> AKWVYKFEEGNASMRNLLGGKGCNLAEMTILGMPIPQGFTVTTEACTEYYNSGKQITQEIQDQIFEAITWLEELNGKKFGDTEDPLLVSVRSAARASMPGMMDTILNLGLNDVAVEGFAKKTGNPRFAYDSYRRFIQMYSDVVMEVPKSHFEKIIDAMKEEKGVHFDTDLTADDLKELAEKFKAVYKEAMNGEEFPQEPKDQLMGAVKAVFRSWDNPRAIVYRRMNDIPGDWGTAVNVQTMVFGNKGETS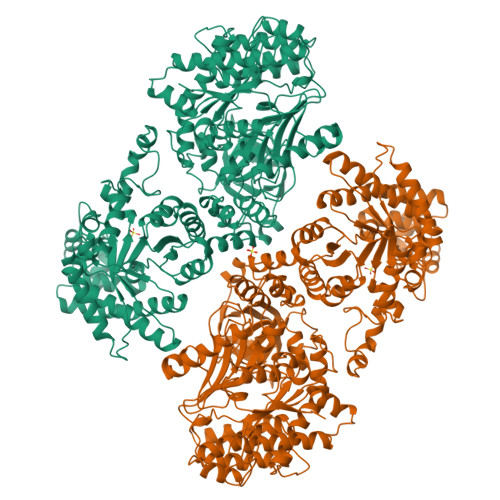GTGVAFTRNPSTGEKGIYGEYLINAQGEDVVAGVRTPQPITQLENDMPDCYKQFMDLAMKLEKHFRDMQDMEFTIEEGKLYFLQTANGKRTAPAALQIACDLVDEGMITEEEAVVRIEAKSLDQLLHPTFNPAALKAGEVIGSALPASPGAAAGKVYFTADEAKAAHEKGERVILVRLETSPEDIEGMHAAEGILTVRGGMTSHAAVVARGMGTCCVSGCGEIKINEEAKTFELGGHTFAEGDYISLDGSTGKIYKGDIETQEASVSGSFERIMVWADKFRTLKVRTNADTPEDTLNAVKLGAEGIGLCRTEHMFFEADRIMKIRKMILSDSVEAREEALNELIPFQKGDFKAMYKALEGRPMTVRYLDPPLHEFVPHTEEEQAELAKNMGLTLAEVKAKVDELHEFNPMMGHRGCRLAVTYPEIAKMQTRAVMEAAIEVKEETGIDIVPEIMIPLVGEKKELKFVKDVVVEVAEQVKKEKGSDMQYHIGTMIEIPRAALTADAIAEEAEFFSFGTNDLTQMTFGFSRDDAGKFLDSYYKAKIYESDPFARLDQTGVGQLVEMAVKKGRQTRPGLKCGICGEHGGDPSSVEFCHKVGLNYVSCSPFRVPIARLAAAQAALNNK>[2x]SNAMAEIKITPEELERIAGNFKNAAGEAQSQINRLEGDINSL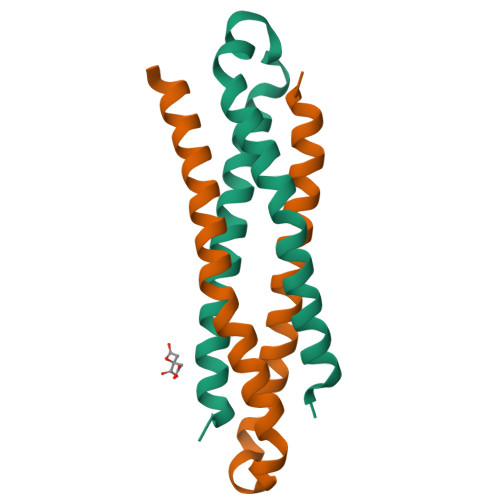EGQWAGATQAKFRGEFIQSKQAMQQFIPILEGISTDLKRIADKFRNTDNAY>DDIKVAVVGAMSGPIAQWGDMEFNGARQAIKDINAKGGIKGDKLVGVEYDDACDPKQAVAVANKIVNDGIKYVIGHLCSSSTQPASDIYEDEGILMISPGATNPELTQRGYQHIMRTAGLDSSQGPTAAKYILETVKPQRIAIIHDKQQYGEGLARSVQDGLKAANANVVFFDGITAGEKDFSALIARLKKENIDFV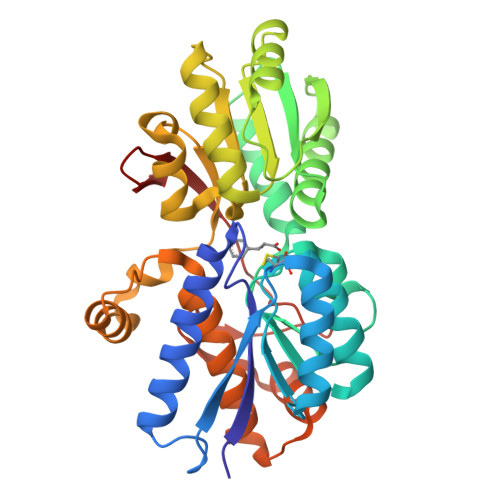YYGGYYPEMGQMLRQARSVGLKTQFMGPEGVGNASLSNIAGDAAEGMLVTMPKRYDQDPANQGIVDALKADKKDPSGPYVWITYAAVQSLATALERTGSDEPLALVKDLKANGANTVIGPLNWDEKGDLKGFDFGVFQWHADGSSTKAK[2x]> GAMDPSAQSSTETFTSKDLFALSYPKSVTRRNDIPEAAASPPSLLSFLRKNVGKDLSSI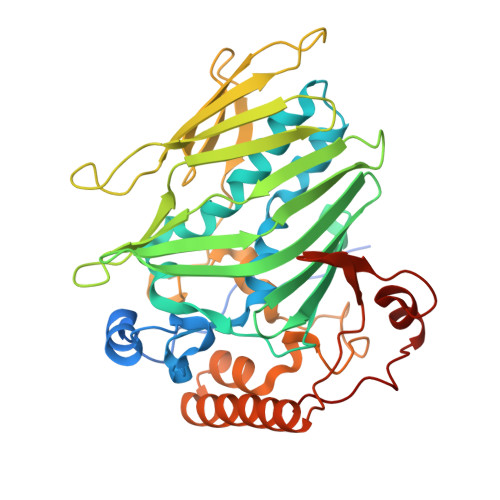AMPVTSNEPISILQLISETFEYAPLLTKATQRPDPITFVSAFAISFLSIYRDKTRTLRKPFNPLLAETFELIREDMGFRLISEKVSHRPPVFAFFAEHLDWECSYTVTPSQKFWGKSIELNNEGILRLKFKTTGELFEWTQPTTILKNLIAGERYMEPVNEFEVHSSKGDKSHILFDKAGMFSGRSEGFKVSIIPPPSSNRKKETLAGKWTQSLANETTHETIWEVGDLVSNPKKKYGFTKFTANLNEITEIEKGNLPPTDSRLRPDIRAYEEGNVDKAEEWKLKLEQLQRERRNKGQDVEPKYFEKVSKNEWKYITGPKSYWERRKKHDWSDISQLW>[10x]SELQTEGRTRYHGRNVCSTWGNFHYKTFDGDVFRFPGLCDYNFASDCRGSYKEFAVHLKRGPGQAEAPAGVESILLTIKDDTIYLTRHLAVLNGAVVSTPHYSPGLLIEKSDAYTKVYSRAGLTLMWNREDALMLELDTKFRNHTCGLCGDYNGLQSYSEFLSDGVLFSPLEFGNMQKINQPDVVCEDPEEEVAPASCSEHRAECERLLTAEAFADCQDLVPLEPYLRACQQDRCRCPGGDTCVCSTVAEFSRQCSHAGGRPGNWRTATLCPKTCPGNLVYLESGSPCMDTCSHLEVSSLCEEHRMDGCFCPEGTVYDDIGDSGCVPVSQCHCRLHGHLYTPGQEITNDCEQCVCNAGRWVCKDLPCPGTCALEGGSHITTFDGKTYTFHGDCYYVLAKGDHNDSYALLGELAPCGSTDKQTCLKTVVLLADKKKNAVVFKSDGSVLLNQLQVNLPHVTASFSVFRPSSYHIMVSMAIGVRLQVQLAPVMQLFVTLDQASQGQVQGLCGNFNGLEGDDFKTASGLVEATGAGFANTWKAQSTCHDKLDWLDDPCSLNIESANYAEHWCSLLKKTETPFGRCHSAVDPAEYYKRCKYDTCNCQNNEDCLCAALSSYARACTAKGVMLWGWREHVCNKDVGSCPNSQVFLYNLTTCQQTCRSLSEADSHCLEGFAPVDGCGCPDHTFLDEKGRCVPLAKCSCYHRGLYLEAGDVVVRQEERCVCRDGRLHCRQIRLIGQSCTAPKIHMDCSNLTALATSKPRALSCQTLAAGYYHTECVSGCVCPDGLMDDGRGGCVVEKECPCVHNNDLYSSGAKIKVDCNTCTCKRGRWVCTQAVCHGTCSIYGSGHYITFDGKYYDFDGHCSYVAVQDYCGQNSSLGSFSIITENVPCGTTGVTCSKAIKIFMGRTELKLEDKHRVVIQRDEGHHVAYTTREVGQYLVVESST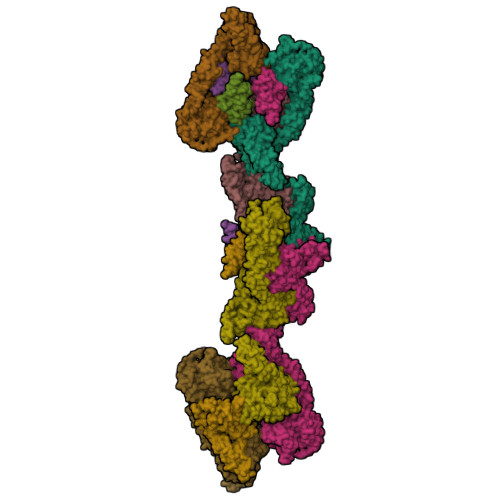GIIVIWDKRTTVFIKLAPSYKGTVCGLCGNFDHRSNNDFTTRDHMVVSSELDFGNSWKEAPTCPDVSTNPEPCSLNPHRRSWAEKQCSILKSSVFSICHSKVDPKPFYEACVHDSCSCDTGGDCECFCSAVASYAQECTKEGACVFWRTPDLCPIFCDYYNPPHECEWHYEPCGNRSFETCRTINGIHSNISVSYLEGCYPRCPKDRPIYEEDLKKCVTADKCGCYVEDTHYPPGASVPTEETCKSCVCTNSSQVVCRPEEGKILNQTQDGAFCYWEICGPNGTVEKHFNICSITTRPSTLTTFTTITLPTTPTSFTTTTTTTTPTSSTVLSTTPKLCCLWSDWINEDHPSSGSDDGDRETFDGVCGAPEDIECRSVKDPHLSLEQHGQKVQCDVSVGFICKNEDQFGNGPFGLCYDYKIRVNCCWPMDKCITHHHHHH>[8x]ASYKVNIPAGPLWSNAEAQQVGPKIAAAHQGNFT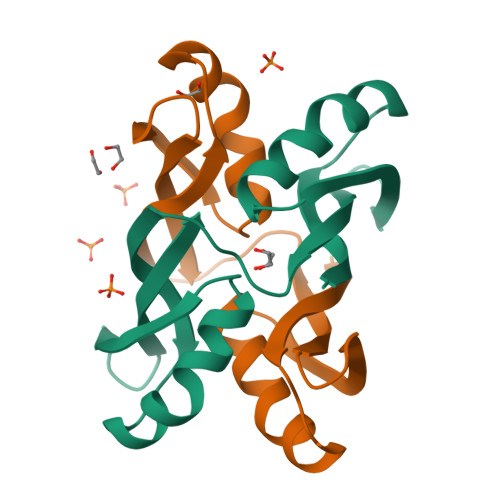GQWTTVVESAMSVVEVELQVENTGIHEFKTDVLAGPLWSNDEAQKLGPQIAASYGAEFTGQWRTIVEGVMSVIQIKYTF> MPTNFTVVPVEARADGAGDEAAERTEEPESPESVDQTSPTPGDGNPRENSPFINNVEVERESYFEGKNMALFEEEMDSNPMVSSLLNKLANYTNLSQGVVEHEEDEDSRRREVKAPRMGTFIGVYLPCLQNILGVILFLRLTWIVGAAGVMESFLIVAMCCTCTMLTAISMSAIATNGVVPAGGSYYMISRSLGPEFGGAVGLCFYLGTTFAGAMYILGTIEIFLTYISPSAAIFQAETADGEAAALLNNMRVYGSCALALMAVVVFVGVKYVNKLALVFLACVVLSILAIYAGVIKTAFAPPDIPVCLLGNRTLANRNFDTCAKMQVVSNGTVTTALWRLFCNGSSLGATCDEYFAQNNVTEIQGIPGVASGVFLDNLWSTYSDKGAFVEKKGVSSVPVSEESRPGGLPYVLTDIMTYFTMLVGIYFPSVTGIMAGSNRSGDLKDAQKSIPTGTILAIVTTSFIYLSCIVLFGACIEGVVLRDKFGEALQGNLVIGMLAWPSPWVIVIGSFFSTCGAGLQSLTGAPRLLQAIARDGIIPFLQVFGHGKANGEPTWALLLTALICETGILIASLDSVAPILSMFFLMCYMFVNLACAVQTLLRTPNWRPRFKFYHWTLSFLGMSLCLALMFICSWYYALFAMLIAGCIYKYIEYRGAEKEWGDGIRGLSLNAARYALLRVEHGPPHTKNWRPQVLVMLNLDSEQCVKHPRLLSFTSQLKAGKGLTIVGSVLEGTYLDKHVEAQRAEENIRSLMSAEKTKGFCQLVVSSNLRDGASHLIQSAGLGGMKHNTVLMAWPEAWKEADNPFSWKNFVDTVRDTTAAHQALLVAKNIDLFPQNQERFSDGNIDVWWIVHDGGMLMLLPFLLRQHKVWRKCRMRIFTVAQVDDNSIQMKKDLQMFLYHLRISAEVEVVEMVENDISAFTYEKTLMMEQRSQMLKQMQLSKNEREREAQLIHDRNTASHTTATARTQAPPTPDKVQMTWTKEKLIAEKHRNKDTGPSGFKDLFSLKPDQSNVRRMHTAVKLNGVVLNKSQDAQLVLLNMPGPPKSRQGDENYMEFLEVLTEGLNRVLLVRGGGREVITIYSSNSLEVLFQ

KCCs are important for K+ and Cl- homeostasis, including in establishing low neuronal cytoplasmic Cl- concentrations critical for inhibitory neurotransmission, and in volume regulation in many cell types. Among KCCs, KCC4 is most strongly activated by cell swelling and high internal [Cl-] and is uniquely active in acidic external environments. KCCs cotransport K+:Cl- in a 1:1 ratio, NKCCs cotransport 1K+:1Na+:2Cl-, and NCCs cotransport 1Na+:1Cl-. Here we report the structure of Mus musculus KCC4 in lipid nanodiscs determined by cryo-EM.

To achieve the highest resolution reconstruction, the nanodisc density was subtracted and particles were subjected to focused classification and subsequent refinement. The resulting map, at 3.65 Å overall resolution, enabled complete de novo modeling of the transmembrane and extracellular region of KCC4 and includes two partial extracellular glycosylation sites, a bound K+ ion, and a bound Cl- ion (Figure 2—figure supplements 5 and 6). KCC4 is monomeric in the nanodisc structure. We conclude that the monomeric structure reported here corresponds to full-length mouse KCC4 with flexible and/or disordered terminal regions. KCC4 is observed in an inward-open conformation that exposes the inside of the transporter to the cytoplasm through a wide and electropositive tunnel that may serve to concentrate the less abundant intracellular substrate Cl-. A prominent feature of KCC4 is a large extracellular domain, unique among proteins of known structure, extending ~35 Å above the membrane. It is formed by EL3 (the long extracellular loop; Hartmann et al., 2010) and EL4, which pack together and cover ~2/3 of the transporter outer surface. In KCC4, residues in EL4, TM1, TM3, and TM10 form an electrostatic and hydrophobic interaction network that seals the gate. The stronger of the two densities between TM1, TM6, and TM3 is modeled as a K+ ion. It is surrounded by electronegative groups contributed by backbone carbonyls (N131 and I132 in TM1 and P429 and T432 in TM6) and a tyrosine hydroxyl from Y216 in TM3. The second site, between TM6 and TM10, is modeled as a Cl- ion.>[2x]MKIYVDGREVIINDNERNLLEALKNVGIEIPNLCYLSEASIYGACRMCLVEINGQITTSCTLKPYEGMKVKTNTPEIYEMRRNILELILATHNRDCTTCDRNGSCKLQKYAEDFGIRKIRFEALKKEHVRDESAPVVRDTSKCILCGDCVRVCEEIQGVGVIEFAKRGFESVVTTAFDTPLIETECVLCGQCVAYCPTGALSIRNDIDKLIEALESDKIVIGMIAPAVRAAIQEEFGIDEDVAMAEKLVSFLKTIGFDKVFDVSFGADLVAYEEAHEFYERLKKGERLPQFTSCCPAWVKHAEHTYPQYLQNLSSVKSPQQALGTVIKKIYARKLGVPEEKIFLVSFMPCTAKKFEAEREEHEGIVDIVLTTRELAQLIKMSRIDINRVEPQPFDRPYGVSSQAGLGFGKAGGVFSCVLSVLNEEIGIEKVDVKSPEDGIRVAEVTLKDGTSFKGAVIYGLGKVKKFLEERKDVEIIEVMACNYGCVGGGGQPYPNDSRIREHRAKVLRDTMGIKSLLTPVENLFLMKLYEEDLKDEHTRHEILHTTYRPRRRYPEKDVEILPVPNGEKRTVKVCLGTSCYTKGSYEILKKLVDYVKENDMEGKIEVLGTFCVENCGASPNVIVDDKIIGGATFEKVLEELSKNG;>MFKNAKEFVQYANKLKTLREKKLNGVSIYVCVGTGCTAKGALKVYSAFEEELKKRNLLGQVTLEKIDDDKVTLNRTGCCGRCSSGPLVKIMPYRFFYSNVAP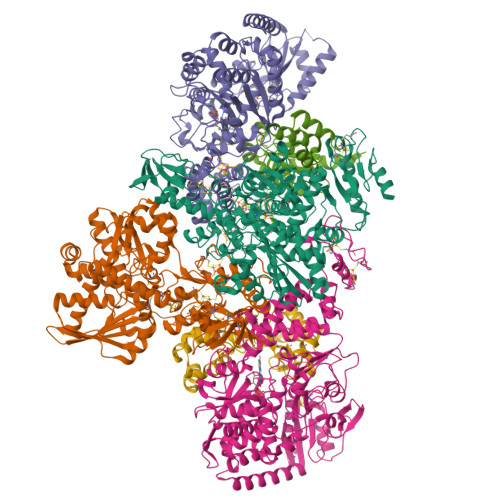EDVPEIVDRTVLKGEPIERLFLTDPLTGEKVPRIEDTTLFKNQDFYIMEAIGESECDSIEDYIARSGYESLVKALTSMTPEEIIETVKASGLRGRGGGGFPTGLKWEFTRKAQGDIKFVVCNGDEGDPGAFMNRTLLERDPHLVLEGMIIAGYAVGAQKGYAYIRAEYPFAVKMFKKAIEDARKLGLLGENILGTGFSFDLEVKEGAGAFVCGEETALLASIEGKRGMPRPKPPFPAQSGLWGKPTLINNVETYANIPRILRDGVENYRKRGTENSPGTKMFSVAGPLKATGIIEVEFGTTLRDIIYNICGGFVEGEEFKAVQIGGPSGACLSEDFIDMPLDYDTLKKADAMVGSGGIVVITKKTCMVEVARFFLDFTKRESCGKCVPCREGTMQAYNILEKFTHGKATYEDLKTLEHLSKTIKTASLCGLGKTAPNPILSTLKLFREEYIAHIEGECPSGMCTAFKKYVINPDICKGCGLCARSCPQNAITGERGKPYTIDQEKCVKCGLCASKCPFKAIELV[2x];>[2x]MASWSHPQFEKSGGGGGENLYFQGAVLALERHFEKVEEILKKYGYKRENLIKILLEIQEIYRYLPEDVINYVSTAMGIPPAKIYGVATFYAQFSLKPKGKYTIMVCDGTACHMAGSPEVLKAIEEETGLTPGNVTEDLMFSLDQVGCLGACALAPVMVINGEVYGNLTADKVKEILRKIKEKERESANV> AGPNRRVIAMPSVRKYAREKGVDIRLVQGTGKNGRVLKE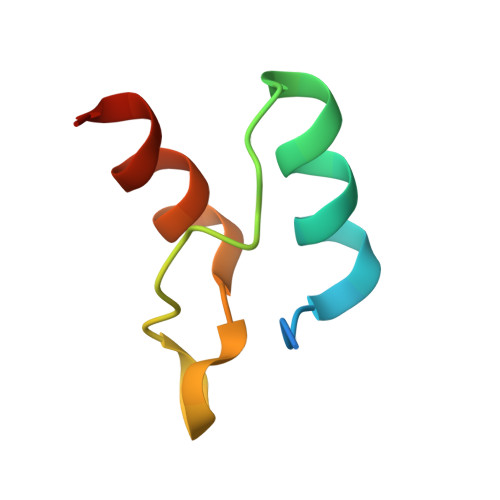DIDAFLAGGA PR-10 refers to a multi-gene family of plant-specific pathogenesis-related proteins of class 10 that are differentially expressed by plants under stressful conditions such as drought, salinity or pathogen invasion. After much debate in the literature about the biological function of these abundant proteins, a consensus seems to be converging on their role in the binding and transport of metabolic mediators such as phytohormones, lipids or flavonoids. Such a ‘molecular container’ view is consistent with the canonical PR-10 fold, which is built around an internal void (cavity) formed by a seven-stranded antiparallel β-sheet curved in a gripping shape around a long C-terminal helix α3. The Hyp-1 protein is important in this context because it has a unique set of three ligand-binding sites consisting of two internal but separated chambers (sites 1 and 2) and a pocket formed by a deep surface invagination (site 3).

When crystallized in the additional presence of melatonin, the Hyp-1–ANS complex formed crystals with a different pattern of structure modulation, in which the supercell shows a ninefold expansion of c, manifested in the diffraction pattern by a wave of reflection-intensity modulation with crests at l = 9n and l = 9n ± 4. Despite complicated tetartohedral twinning, the structure has been successfully determined and refined to 2.3 Å resolution using a description in a ninefold-expanded supercell, with 36 independent Hyp-1 chains and 156 ANS ligands populating the three internal (95 ligands) and five interstitial (61 ligands) binding sites. A similar association is observed in the present structure, where dimers are created by antiparallel association of the β1 strands of adjacent protein molecules. The characteristic zigzag pattern of the two columns in the unit cell is the result of the noncrystallographic 21/9 screw-axis operation, which combines an ∼180° rotation with an ∼1/18 translation along the screw axis in the direction. In Hyp-1 this internal cavity is divided into two distinct chambers, 1 and 2, with a separating partition (Arg27) and separate entrances, E1 and E2, respectively. Stabilization of ligand molecules in chamber 1 occurs mainly through hydrogen-bond formation between Arg27 and the sulfonate group of ANS. Site 3 is created by stacking interactions, with the ligand molecule held in place between the jaws (Tyr150 from helix α3 and Lys33 from helix α2) of a molecular vise. The ANS ligands in the superficial sites 4, 5 and 6 concatenate adjacent protein chains into a unique helical pattern. Furthermore, other buffer-solution molecules (sulfate, HEPES, citrate and dimethyl sulfoxide) were found in the structure at selected ligand-binding sites that are typically reserved for ANS.

>[36x]DPFTMAAYTIVKEEESPIAPHRLFKALVLERHQVLVKAQPHVFKSGEIIEGDGGVGTVTKITFVDGHPLTYMLHKFDEIDAANFYCKYTLFEGDVLRDNIEKVVYEVKLEAVGGGSKGKITVTYHPKPGCTVNEEEVKIGEKKAYEFYKQVEEYLAANPEVFA>MIDFLKQLPHLEPYGNPFYFIYLGIALLPIFIGLFFKKRFAIYECLVSITFIVLALTGTHASQILALLFYIVWQIIWVYSYKRYRSQRDNKWVFYLHSFLVVLPLILVKVEPTINGTQSLLNFLGISYLTFRAVGMIIEMRDGVLKEFTLGEFLRFMLFMPTFTSGPIDRFKRFNEDYQSIPNRDELLNMLEQAVKYIMLGFLYKFVLAQIFGSMLLPPLKAQALSQGGIFNLPTLGVMYVYGFDLFFDFAGYSMFALAVSNLMGIKSPINFDKPFISRDMKEFWNRWHMSLSFWFRDFVFMRL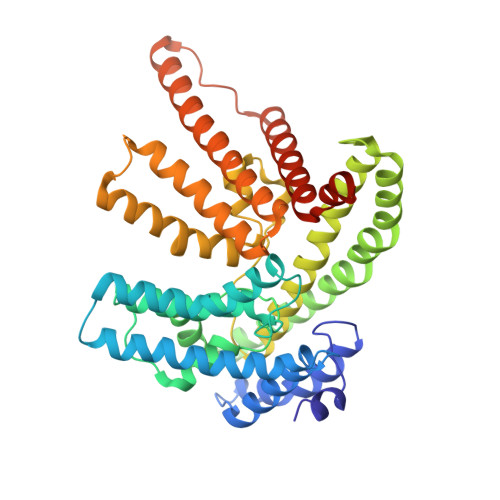VIVLMRNKVFKNRNTTSNVAYIINMMVMGFWHGITWYYIAYGIFHGIGLVINDAWLRKKKTINKDRKKAGLKPLPENKWTKALGIFITFNTVMLSFLIFSGFLNDLWFTKKLEHHHHHHHH[4x]>[3x]GSHMPGPVARLAPQAVLTPPSAASLFLVLVAGDSDDDRATVCDVISGIDGPLKAVGFRELAGSLSCVVGVGAQFWDRVSASSKPAHLHPFVPLSGPVHSAPSTPGDLLFHIKAARKDLCFELGRQIVSALGSAATVVDEVHGFRYFDSRDLLGFVDGTENPTDDDAADSALIGDEDPDF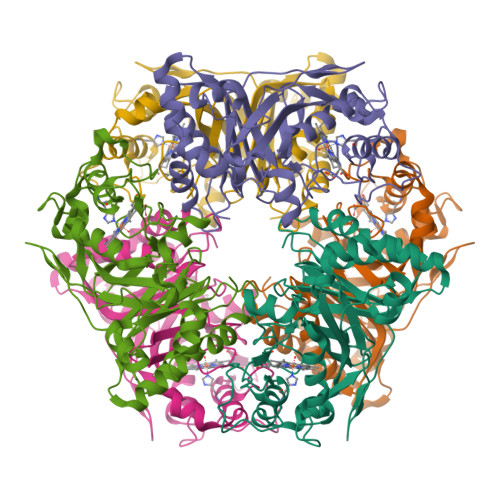RGGSYVIVQKYLHDMSAWNTLSTEEQERVIGRTKLENVELDDDAQPSNSHVTLNTIVDDDGVEHDILLDNMAFGSLGEAEYGTYFIGYAKDPAVTELMLRRMFLGEPPGNYDRVLDFSTAATGTLFFVPSRDVLESLGDEPAGAESAPEDPVEPAAAGPYDLSLKIGGLKGVSQ>[4x]MTMDTAQLKSQIQQYLVESGNYELISNELKARLLQEGWVDKVKDLTKSEMNINESTNFTQILSTVEPKALEMVSDSTRETVLKQIREFLEEIV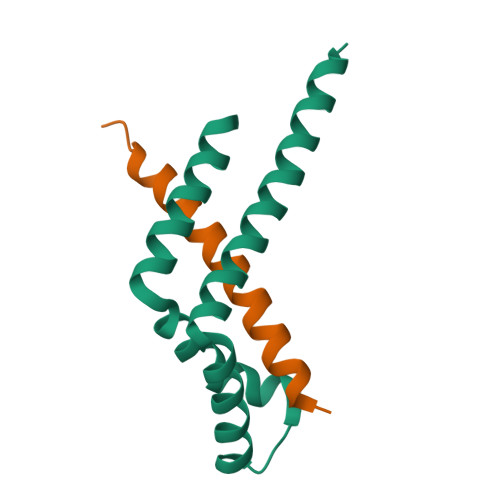DTQ;>TEETITIDSISNGILNNLLTTLIQDIVARETT[4x]> SKVLVLKSSILAGYSQSNQLSDYFVEQWREKHSADEITVRDLAANPIPVLDGELVGALRPSDAPLTPRQQEALALSDELIAE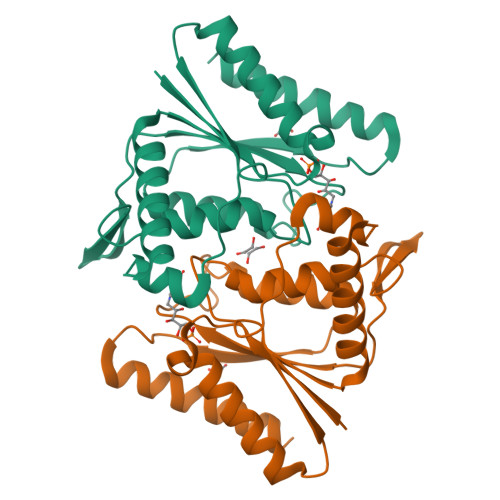LKAHDVIVIAAPMYNFNISTQLKNYFDLVARAGVTFRYTENGPEGLVTGKKAIVITSRGGIHKDGPTDLVTPYLSTFLGFIGITDVKFVFAEGIAYGPEMAAKAQSDAKAAIDSIVSA> GSPDPRAELDSTVLLTRSLLADTRQLAAQLRDKFPADGDHNLDSLPTLAMSAGALGALQLPGVLTRLRADLLSYLRHVQWLRRAGGSSLKTLEPELGTLQARLDRLLRRLQLLMSRLALPQPPPDPPAPPLAPPSSAAGGIRAAHAILGGLHLTLDWAVRGLLLLKTRL

Interleukin (IL-), an IL-6 family cytokine, has pivotal roles in autoimmune diseases, fibrotic complications, and solid cancers. IL-11 activates downstream signalling pathways by binding its two cell surface receptors: the IL-11 specific receptor, IL-11Rα, and the signal-transducing receptor, glycoprotein (gp)13013,26. Following the formation of the receptor complex, the Janus kinase (JAK)/signal transducer and activator of stat (STAT) and extracellular signal regulated kinase (ERK)/mitogen-activated protein kinase (MAPK) pathways are primarily activated. IL-11 and IL-6 utilise a homodimer of gp13026,34,35 while other IL-6 family members exploit a heterodimer of gp130 with a second signal-transducing receptor, such as LIF receptor (LIFR), OSM receptor (OSMR), IL-27R/WSX-1 or IL-12 receptor β−2 subunit (IL-12Rβ2).

We solved crystal structures of IL-11Δ10/Mutein and IL-11Δ10/W147A at resolutions of 1.8 Å and 1.5 Å, respectively, to understand the structural consequences of the mutations. SAXS experiments show that the crystal structures are representative of the solution structure, and SV-AUC indicates that both proteins are monomeric in solution. The structure of IL-11Δ10/W147A is similar to the structure of IL-11Δ10 (RMSD 0.3 Å relative to IL-11Δ1049), indicating that the W147A mutation does not alter the structure. Thus, the 58PAIDY62 mutations alter the position of the AB-loop, shifting the register of key loop-core interactions by three residues, while maintaining the composition of the interacting residues. This register change is due to a shift of the LX(S/T)LP motif that mediates loop-core contacts: In IL-11Δ10 and IL-11Δ10/W147A the motif is 51LDSLP55, while in IL-11Δ10/Mutein the interacting motif is 54LPTLP58. Conversely, stimulation with IL-11Δ10/Mutein alone does not result in STAT3 activation, demonstrating that the mutations eliminate the ability of IL-11Δ10/Mutein to signal, in agreement with previous reports. Surprisingly, stimulation with either IL-11Δ10/W147A or IL-11Δ10/PAIDY resulted in robust STAT3 activation, albeit with a higher EC50 than IL-11Δ10, of 610 ± 120 pM (p = 0.04 vs IL-11Δ10) and 140 ± 12 pM (p = 0.01 vs IL-11Δ10), respectively. However, a small population of hexameric complex at ~7.5 S was observed in the sedimentation coefficient distributions, indicating that the W147A mutation alone permits some hexamer formation and consistent with the ability of IL-11Δ10/W147A to stimulate STAT3 activation in vitro. In contrast, neither IL-11Δ10/W147A or IL-11Δ10/PAIDY inhibited IL-11Δ10 mediated STAT3 activation, contradicting previous reports that the W147A mutation alone is an effective IL-11 signalling inhibitor.>SNAQDQ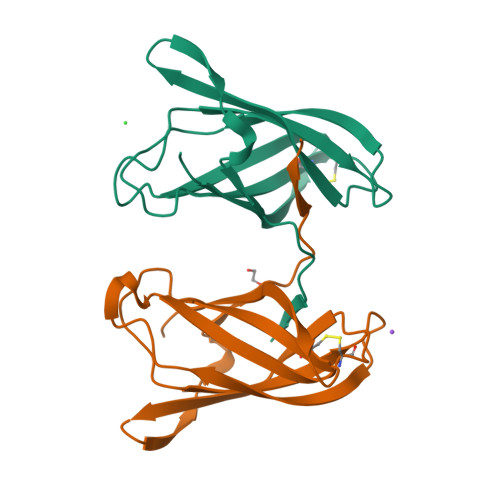RYISIRNTDTIWLPGNICAYQFRLDNGGNDEGFGPLTITLQLKDKYGQTLVTRKMETEAFGDSNATRTTDAFLETECVENVATTEIIKATEESNGHRVSLPLSVFDPQDYHPLLITVSGKNVN[2x]> MEGERKNNNKRWYFTREQLENSPSRRFGVDPDKELSYRQQAANLLQDMGQRLNVSQLTINTAIVYMHRFYMIQSFTQFPGNSVAPAALFLAAK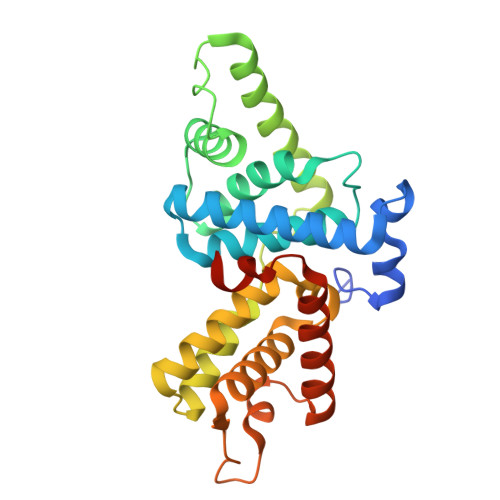VEEQPKKLEHVIKVAHTCLHPQESLPDTRSEAYLQQVQDLVILESIILQTLGFELTIDHPHTHVVKCTQLVRASKDLAQTSYFMATNSLHLTTFSLQYTPPVVACVCIHLACKWSNWEIPVSTDGKHWWEYVDATVTLELLDELTHEFLQILEKTPNRLKRIWNWRACEAA> TGLAADIRWTAYGVPHIRAKDERGLGYGIGYAYARDNACLLAEEIVTARGERARYFGSEGKSSAELDNLPSDIFYAWLNQPEALQAFWQAQTP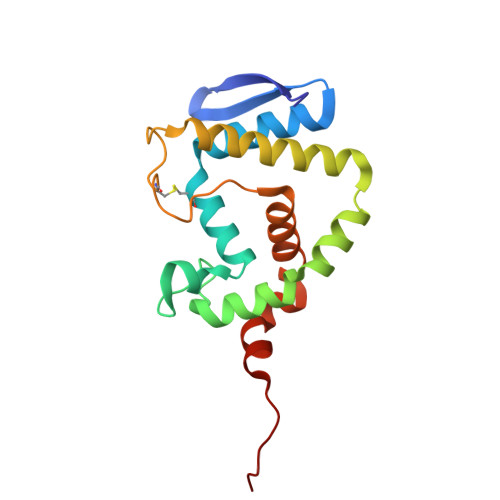AVRQLLEGYAAGFNRFLREADGKTTSCLGQPWLRAIATDDLLRLTRRLLVEGGVGQFADALVAAAPPGAEK>[4x]CGGACCGAGCCAG;>[4x]GCU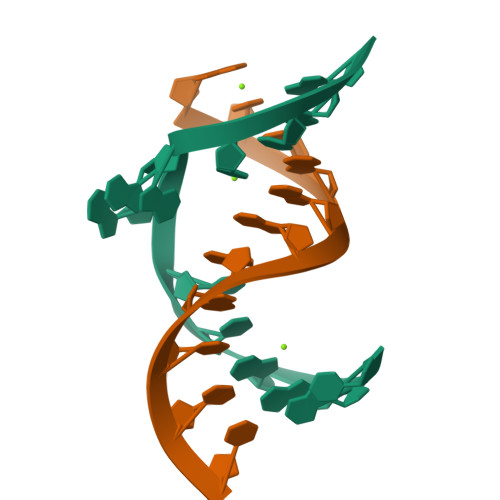GGGAGUCC Host proteases, TMPRSS2 and CTSL/CTSB cleave the SARS-CoV-2 spike to play a crucial role in the two alternative pathways of viral entry and are characterized as promising pharmacological targets. The entry of SARS-CoV-2 depends on two distinctive pathways, cell surface entry and endosomal entry, where the transmembrane serine protease, TMPRSS2, and endosomal cysteine proteases cathepsin L/B (CTSL/CTSB) cleave the viral spike protein. The crystal structures of TMPRSS2 and CTSL/CTSB in complex with the potent inhibitors were determined to reveal their specific mode of interaction.

Nafamostat and camostat, two clinically available drugs used to treat pancreatitis, displayed excellent inhibitory potency with IC50 values of 0.40 nM and 9.00 nM, respectively. The crystal structures of TMPRSS2 in complex with nafamostat, camostat, and UK-371804, were determined to 2.6 Å, 2.4 Å and 2.6 Å, respectively. Initially, they bind to TMPRSS2, forming the Michaelis complex. The ester group in their common guanidinobenzoyl moiety then reacts with the catalytic serine of TMPRSS2 to form the acyl-enzyme intermediate and cleave off the “leaving group”. The guanidinobenzoyl group stays covalently linked to the catalytic serine and disables the protease activity. Our structures of TMPRSS2 in complex with nafamostat and camostat both capture the post-reaction state, leaving the identical remnant moiety in the catalytic site of the SP domain. Apart from the ester bond formed with γO of the catalytic serine, the guanidyl head of the guanidinobenzoyl moiety forms a salt bridge with Asp435, and is further anchored by hydrogen bonds with Ser436 and Gly464 in the S1 pocket. The crystal structures of TMPRSS2 in complex with nafamostat or camostat in our study, and a previously reported structure of TMPRSS2 in complex with nafamostat, demonstrate a high degree of similarity, with the r.m.s.d values ranging from 0.296 to 0.445 Å for all Cα atoms of their SP domains (residues 256–492). The values are low because only the same remnant moiety of guanidinobenzoyl group occupies the active site of TMPRSS2 after the reaction, although the complete structures of nafamostat and camostat are different.

>[2x]MGSKCSNSGIECDSSGTCINPSNWCDGVSHCPGGEDENRCVRLYGPNFILQVYSSQRKSWHPVCQDDWNENYGRAACRDMGYKNNFYSSQGIVDDSGSTSFMKLNTSAGNVDIYKKLYHSDACSSKAVVSLRCIACGVNLNDDDDK;>IVGGESALPGAWPWQVSLHVQNVHVCGGSIITPEWIVTAAHCVEKPLNNPWHWTAFAGILRQSFMFYGAGYQVEKVISHPNYDSKTKNNDIALMKLQKPLTFNDLVKPVCLPNPGMMLQPEQLCWISGWGATEEKGKTSEVLNAAKVLLIETQRCNSRYVYDNLITPAMICAGFLQGNVDSCQGDSGGPLVTSKNNIWWLIGDTSWGSGCAKAYRPGVYGNVMVFTDWIYRQMRADGEFVEHHHHHHHH[2x]>GADLADRFAELERRYDARLGVYVPATGTTAAIEYRADERFAFCSTFKAPLVAAVLHQNPLTHLDKLITYTSDDIRSISPVAQQHVQTGMTIGQLCDAAIRYSDGTAANLLLADLGGPGGGTAAFTGYLRSLGDTVSRLDAEEPELNRDPPGDERDTTTPHAIALVLQQLVLGNALPPDKRALLTDWMARNTTGAKRIRAGFPAD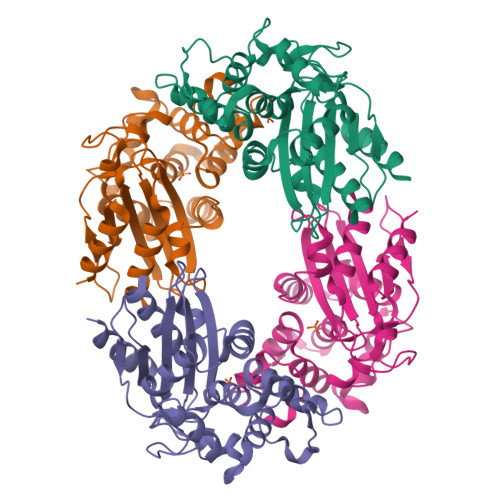WKVIDKTGTGDYGRANDIAVVWSPTGVPYVVAVMSDRAGGGYDAEPREALLAEAATCVAGVLA[4x]>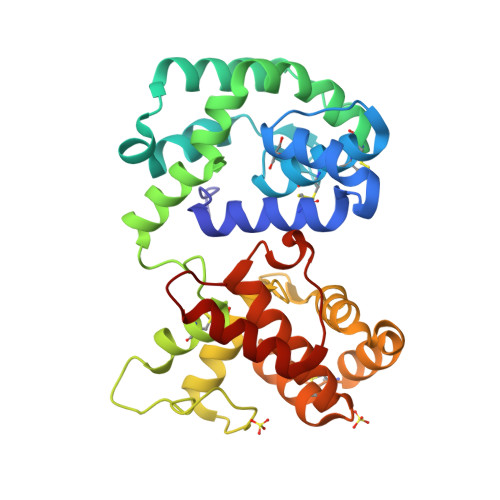 QPWKALDAEQALYVYKRCYEDHLPSGSDRKTYMTLWNAWRLEPNDAITHCYAKCVLTGLQIYDPQENAFKSDRIPVQYQAYKTITQSKQKEVTEYQKALAAANAKSGSCVDLYNAYLPVHNRFVNLSRQLYHGTVEGAAKIYAAMPEIKQKGESFHAYCEKRAWKGNKQSEWKNGRRYKLTGSPELKDAIDCIFRGLRYMDDTGLKVDEIVRDFNLINKSELEPEVRSVLASCKGSEAYDYYVCLVNSRLKQHFKNAFDFHELRSADYAYLLRGKVYENPEKVKEEMKKLNTTVHF Modified form of Cinnamtannin B1 with sp3 hybridized 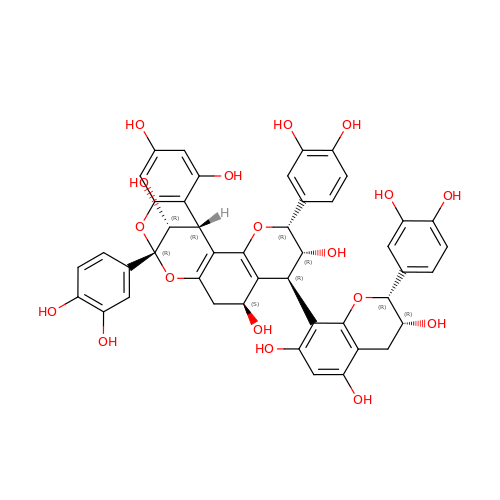C5' | C45 H38 O18 | GTLDPRJUMQNNPF-PUHQMIONSA-N> LPRRLHLEPAFLPYS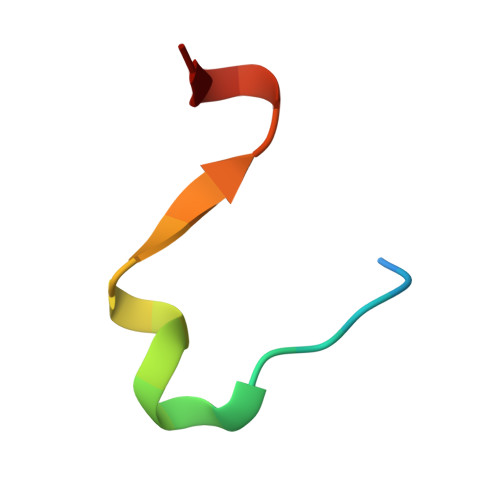VKAHECC>MTKIAL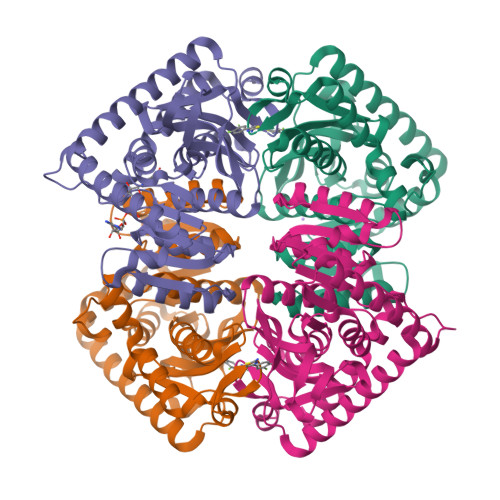IGSGQIGAIVGELCLLENLGDLILYDVVPGIPQGKALDLKHFSTILGVNRNILGTNQIEDIKDADIIVITAGVQRKEGMTREDLIGVNGKIMKSVAESVKLHCSKAFVICVSNPLDIMVNVFHKFSNLPHEKICGMAGILDTSRYCSLIADKLKVSAEDVNAVILGGHGDLMVPLQRYTSVNGVPLSEFVKKNMISQNEIQEIIQKTRNMGAEIIKLAKASAAFAPAAAITKMIKSYLYNENNLFTCAVYLNGHYNCSNLFVGSTAKINNKGAHPVEFPLTKEEQDLYTESIASVQSNTQKAFDLIKAAALEHHHHHH[4x]>[3x]HHHHHHMQLRFARLSEHATA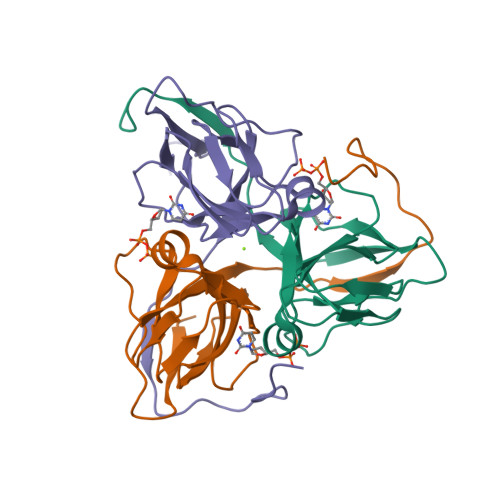PTRGSARAAGYDLYSAYDYTIPPMEKAVVKTDIQIALPSGCYGRVAPRSGLAAKHFIDVGAGVIDEDYRGNVGVVLFNFGKEKFEVKKGDRIAQLICERIFYPEIEEVQALDDTERGSGGFGSTGKN> LPSFVDWRSKGAVNSIKNQKQCGSCWAFSAVAAVESINKIRTGQLISLSEQELVDCDTASHGCNGGWMNNAFQYIITNGGIDTQQNYPYSAVQGSCKPYRLRVVSINGFQRVTRNNESALQSAVASQPVSVTVEAAGAPFQHYSSGIFTGPCGTA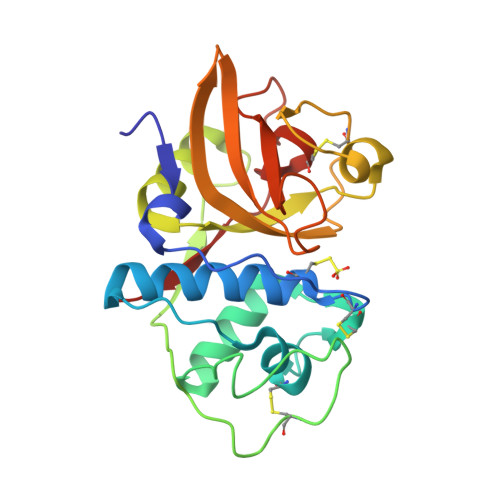QNHGVVIVGYGTQSGKNYWIVRNSWGQNWGNQGYIWMERNVASSAGLCGIAQLPSYPTKA> SKKIGLFYGTQTGKTESVAKIIRDEFGNDVVTLHDVSQAEVTDLNDYQYLIIGCPTWNAGELQSDWEGLYSKLDDVDFNGKLVAYFGTGDQAGYADNFQD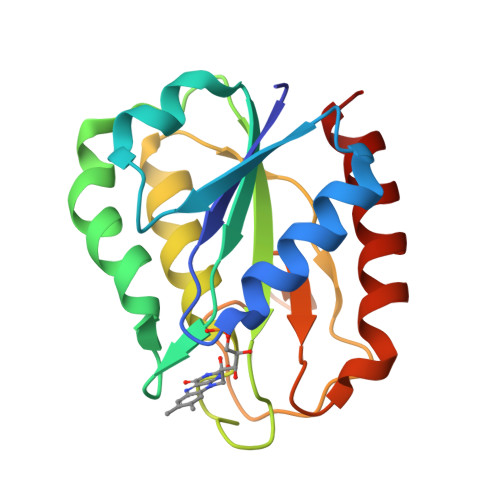AIGILEEKISQRGGKTVGYWSTDGYKFNDSKALRNGKFVGLVLDEDNQSDLTDDRIKSWVAQLKSEFGL>PLIAAASVIAAGLAVGLASIGPGVGQGTAAGQAVEGIARQPEAEDKIRGTLLLSLAFMEALTIYGLVVALALLFANPFV[14x]

ATP (adenosine tri-phosphate), the general energy currency of the cell, is supplied mainly by FOF1-ATPase (ATP synthase). This enzyme is composed of two rotary machines, FO and F1, which are coupled by a central rotor and a peripheral stator. A homo-oligomeric ring of the hairpin-shaped subunit c is included in the Fo domain. The c-ring of the enzyme's CFo portion consists of 14 copies of subunit c, and is embedded in the membrane.

We isolated the c-ring of the FOF1-ATPase of the green pea (Pisum sativum) from a native preparation, crystallized it, and determined its homo-tetradecameric structure at a resolution of 3.4Å. The crystal structure of the c-ring from P. sativum shows a concave barrel shape with a pronounced waist in the middle, exhibiting tetradecameric symmetry consisting of an inner and an outer ring. Each monomer was a hairpin-shaped, 81-residue polypeptide, containing two trans-membrane (TM) helices; TM1 (residues 4–41) composed the inner ring, and TM2 (residues 46–75) formed the outer ring. The proton-binding site retains a chemical coordination similar to that of the alkalophilic cyanobacterium Spirulina platensis, including the same amino acids: Gln28 and Glu61, located on TM1 and TM2, respectively, of the same monomer, and Phe59 and Tyr66, which are positioned on TM2 of an adjacent monomer. The Oε2 part of the carboxyl group of Glu61 generates hydrogen bonds with the Nε2 of Gln28 and the carbonyl group of Phe59 (with distances between relevant atoms of 3.1Å and 2.8Å, respectively). The second oxygen group, Oε1, forms a hydrogen bond with the hydroxyl group of Tyr66 (2.9Å). This chemical coordination represents a locked conformation of the binding site. Glu61 is likely to be protonated in the structure, which was crystallized at pH 4.5, and this notion is supported by a pKa analysis. One contact region consisted of loop-to-loop interactions mediated by yttrium ions, as indicated by strong electron densities. A galactolipid was tentatively modeled into the intercalating electron density, in compliance with the notion that the uncharged heads of the galactolipids enable their penetration through the thylakoid membrane, as was demonstrated in the crystal structure of cyanobacterial photosystem II.>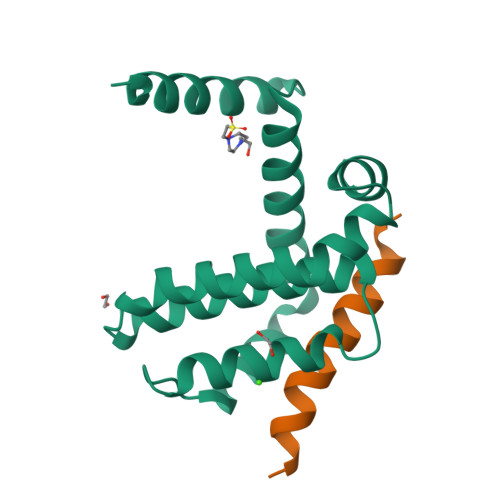GPLGSMSQSNRELVVDFLSYKLSQKGYSWSQMAAVKQALREAGDEFELRYRRAFSDLTSQLHITPGTAYQSFEQVVNELFRDGVNWGRIVAFFSFGGALCVESVDKEMQVLVSRIAAWMATYLNDHLEPWIQENGGWDTFVELYGNNAAAESRKGQER[2x];>EVIPMAAVKQALREAGDEFELRYR[2x]> ALYINDDCTACD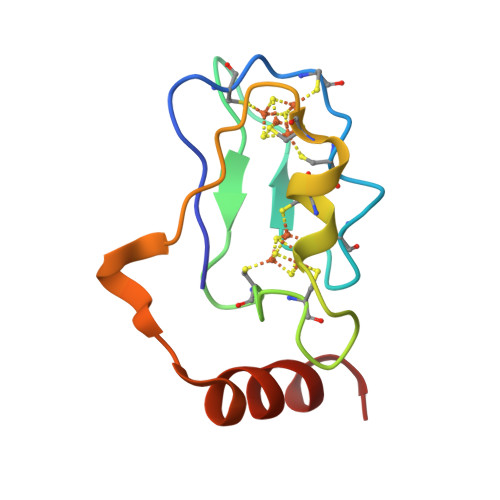ACVEECPNEAITPGDPIYVIDPTKCSECVGAFDEPQCRLVCPADCIPDNPDYRETREELQEKYDRLHG>PSDKPVAHVVANPQAEGQLQWSNRRANALLANGVELRDNQLVVPIEGLFLIYSQVLFKGQGCPSTHVLLTHTISRIAVSYQTKVNLLSAIKSPCQRETPEGAEAKPWYEPIYLGGVFQLEKGDRLSAEINRPDYLDFAESGQVYF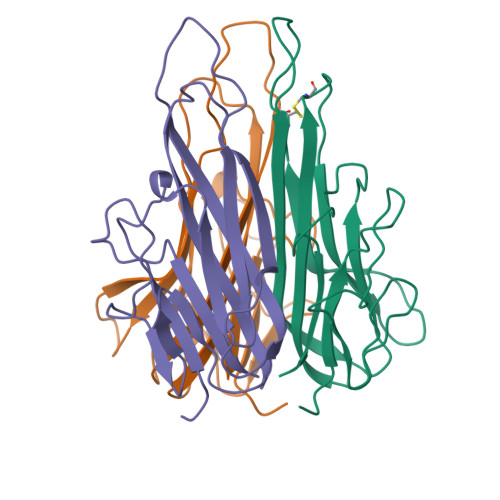GIIAL[6x]>MKLEQQIQRVILEEAKALIKDYHEYHNRVHLESVRNKKRLGDSAPDKKIHRPNYWSFDKKFDPFYVKSNYKSIARSIANKIENRTYLPNEPFTKDVPKPDGGIRKVSIYQIPDAAISKLFFNRLLAKNRHRFSSFSYAYRNDRNVHFAIQDISVDLKKNERTFLAEFDFSDFFGSISHSFLNEQFNENGFYISPEEKFIIRSFLRERKVGIPQGTSISLFLANLTCWKLDQDLEREGVKFSRYADDTIIWSQEYSKICNAFNIITNFSKSAGIKINPKKSEGISLLTKKGLPSEITSKNNL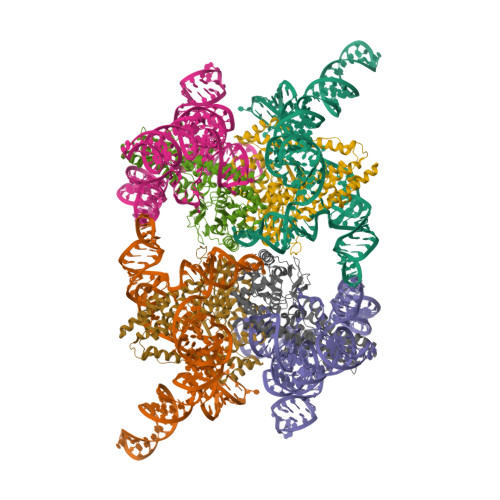DFLGYTLSVENVSIKEKSVKKIKKQISYILYRNLIQPLKKTSLAGQTIPANDRDKNFLIAICEIRRYMYGGLSKSQIKDYLSGRSNRLYFKGIMSFYPLVNDVEQLKQLDGWIVSVIYRALKLRCQLLSKWGYNRSHNFPFILDREDIVDKCSKKTIAGRKLFEIPSFLLIHKALQKGLQESGIEKIMNPQSLNYDYE[4x]> FELLVSFLNTPKYGTFDPTPVVPVFFPFWFGMIVGDIGYALLFYLVGRWLSGYVKRNEPLVIDLFALKLKPQVIGKLVHILNWMVFWTVVWGVIYGEFFGTFLEHLGVFGTPEHPGLIPILIHRIDTAKTANLLILLSVAFGVVLVFFGLALRAYLGLKHRHMAHFWEGVGYLGGLVGVLALAASYLGNLQAGWLQGLMYLGFGVFLLAVLMSRIWLMIPEIFTQAGHILSHIRIYAVGAAGGILAGLLTDV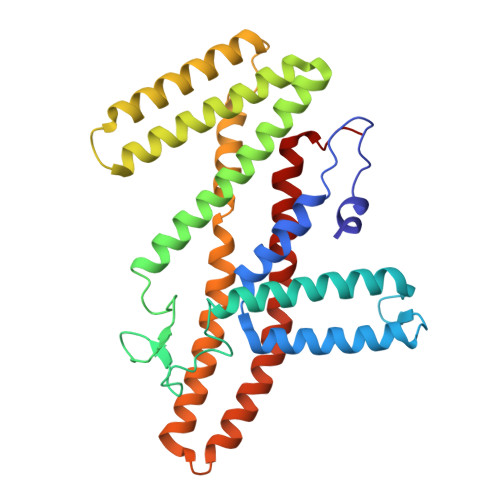GFALAERLGLLGVLLGLLVAGVLHLLILLLTTLGHMLQPIRLLWVEFFTKFGFYEE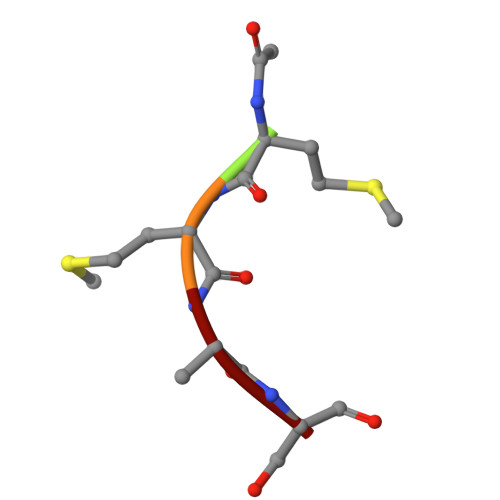> XMMAS>[2x]MAGLSVSDHLDGQLARLCEVAGADPVEPRNLLAGLLGPVGPRPLYEPPAWPSGVSDDHTPVEFSIAFNEAEPPTLRILGETLGSPP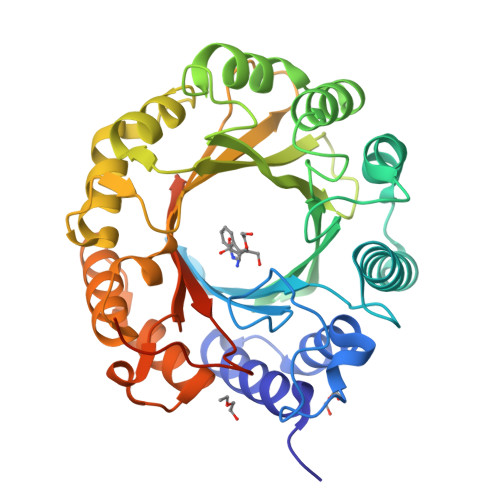GPLANLSATRGFLDAQARRAGLSTSRLDSVRDLFATDDPQGDFAMWCSLVFRSSRRPEFKVYLNPEVKGVERSPALVSEALHRLGLGASYRALLDHGVRPGELGRGDRLTFFAVDLHDGPQARVKLYLTHHEAEVWDVTRAASVVDGVDVAEIEEFCVVAGGGTRRFDGRPLVGSYTFTEGADRPVGYSIYVPIRSYVTDDQEARDRVAALLVRYGFDTDGLDRAIAAVTPRPLRDGVGLIAHVSLRLGAPRPGVTVYLSAEAYRVSPPRPRLVPRGSSHHHHHHHH The B antigen that is present on red blood cells (RBCs) of type B only differs from the H antigen that defines type O by the terminal galactose unit connected by an α‐1,3‐glycosidic bond to the sub‐terminal galactose. Thus, removal of this additional galactose yields the H antigen of blood type O. For this, we characterized several previously unstudied α‐1,3‐galactosidases belonging to the GH110 family. Our findings revealed that the α‐1,3‐galactosidase from Pedobacter panaciterrae (PpaGal) exhibits superior efficiency compared to previously described galactosidases. Analysis of the structures revealed that the core β‐helix of PpaGal is surrounded by two small β‐barrel domains (domains I and II) as it is typical for enzymes of the GH110 family.

Since crystallization approaches with PpaGal constructs containing a N‐terminal His‐tag were not successful (data not shown), a TEV‐protease‐cleavage site was introduced via site‐directed mutagenesis enabling to remove the His‐tag after purification. Indeed, after His‐tag removal, several crystals were obtained and two structures were solved. The structure of PpaGal in complex with galactose was refined to 2.98 Å resolution, while a resolution of 2.75 Å was obtained for the structure of the non‐complexed apo‐form of PpaGal. Additionally, a stacking geometry via CH‐π‐interaction between the galactose and the tryptophan W497 was found, which often occurs in CAZymes. Interestingly the position of this tryptophan residue shifts if no galactose is bound. Therefore, this specific tryptophan residue which is also highly conserved, seems to have a “gating function” for the substrate. Furthermore, two crystal structures of PpaGal in its galactose free and galactose‐bound state were solved.

>[4x]SEFNVKIYKLSAYGIKPNSGKNTTPLLTSLLKEIKSKTSDLDKVIIQFEKGRYDFYPEGAIKREYYISNHDQDNPKTVGIGIEKFNNITLIGKGTDLMFHGRMLPLALIESSNVKIKDLNIDFEKPQITQVKIISNDTTAGNIVFETAPWVKYKLKDSTFYNTGEGWEMQPTSGIAFENGTKHIIFNSGDIGVGTKSVSEVSPGKIMAHHWKNKKLVPGTVIAMRSWQRPAPGIFVHKGKNISFENVKVHYAEGMGLLAQLTENIYMDGFGVCLRGKNDPRYFTTQADATHFSGCKGEIVSKNGLYEGMMDDAINIHGTYLKITKKLDDHTVIANYMHEQSYGFDWGNIRDTVQFIQSKTMELWDAKNTIASIKPILRNSTDPIKEFRIEFTKALDPVIDPSKQDIGIENLSWTPSVVFTGNTIRNNRARGALFSTPKPTLVANNLFDHTSGCAILLCGDSNGWYETGSCRDITIRDNKFVNALTSMYQFTSAIISIYPEIPDLTNQKKYFHSGIRILNNQFDTFDQPILYAKSVDGLVFTGNKIQTNKEYPAFHSNKKRFLFERVIGVDFSDNKVDGKPIEML> GSHMADKELKFLVVDDFSTMRRIVRNLLKELGFNNVEEAEDGVDALNKLQAGGYGFVISDWDMPN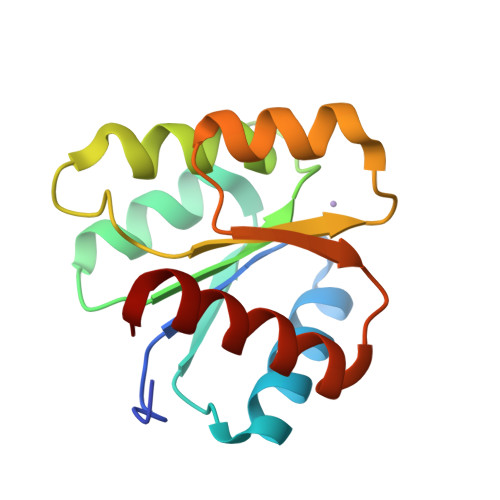MDGLELLKTIRADGAMSALPVLMVTAQAKKENIIAAAQAGASGYVVKPFTAATLEEKLNKIFEKLGM>GGPGNEKLKEKENNDSSDKATVIPNFNTTMQGSLLGDDSRDYYSFEVKEEGEVNIELDKKDEFGVTWTLHPESNINDRITYGQVDGNKVSNKVKLRPGKYYL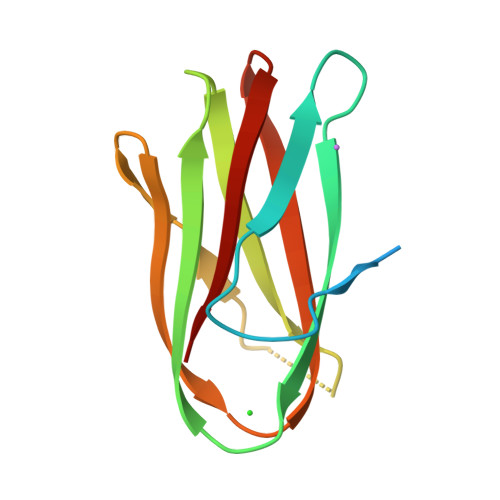LVYKYSGSGNYELRVNK[2x]>[2x]DMPVERILEAELAVEPKTETYVEANMGLNPSSPNDPVTNICQAADKQLFTLVEWAKRIPHFSELPLDDQVILLRAGWNELLIA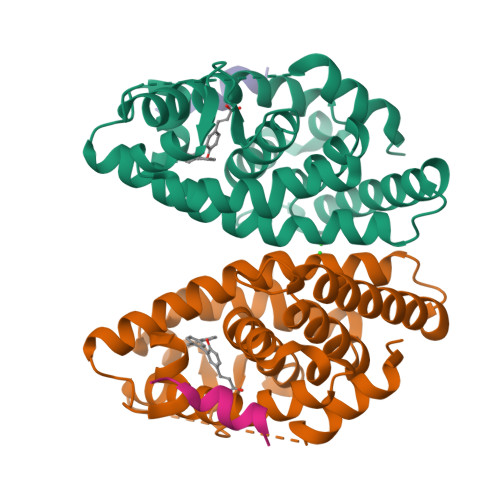SFSHRSIAVKDGILLATGLHVHRNSAHSAGVGAIFDRVLTELVSKMRDMQMDKTELGCLRAIVLFNPDSKGLSNPAEVEALREKVYASLEAYCKHKYPEQPGRFAKLLLRLPALRSIGLKCLEHLFFFKLIGDTPIDTFLMEMLEA;>KHKILHRLLQD[2x]> INIGNKTNENVISFFDSTDAETQNHNALMKGCGEFIVNLRTLLRTFRTITDNWILQANTKTPITDLTNTTDAQGRDYMSYLSYLYRFYRGGRRYKFFNTTPLKQSQTCYIRSFLIPRNYSADEINVDGPSHITYPVINPVHEVEVPFYSQYRKIPIASTSDKGYDSSLMYFSNT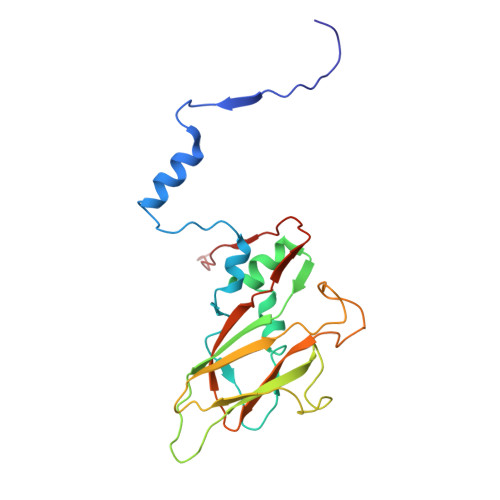ATTQIVARAGNDDFTFGWMIGPPQLQGESRSVAP>PIIQMNLLEGRTVEQKRNAVAAITEAVVRTLDVRPD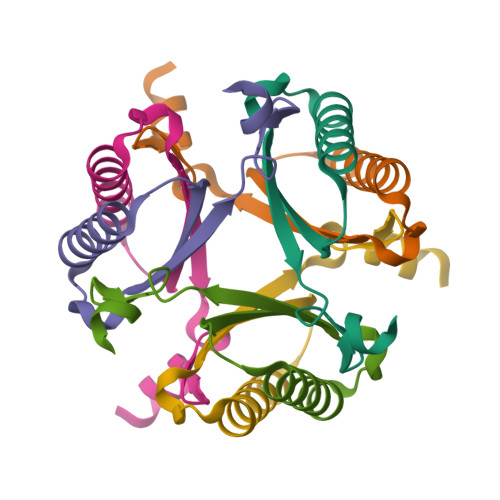QVRILINELGVEHFSVAGQTAAMRQAAAANAKDL[2x]> PTYVDPSKCDGCKGGEKTACMYICPNDLMILDPEEMKAFNQEPEACWECYSCIKICPQGAITARPYADFAPMGGTCIPLRGSEDIMWTIKFRNGSVKRFKFPIRTTPEGSIKPFEGKPEAGDLENELLF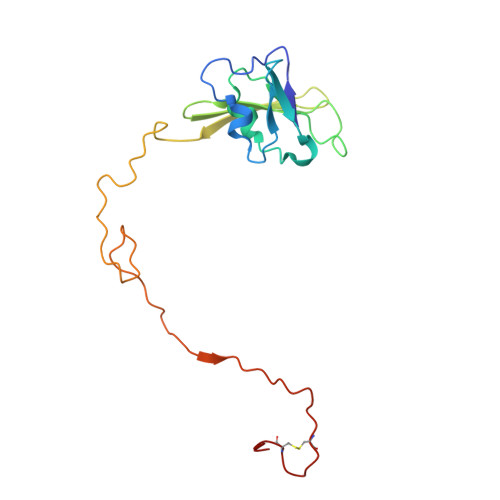TETALTVPQVALGQKAQIADAETSQCWFDLPCEGGNR>HHNKVRTCWNEGRPALAGWLQLPGTLHAEALARLDYDAVVIDMQHSPIDFGQVAPMLIAIELGGAEPFVRTQVNDPSDIMKLLDAGAYGIIAPMVNTRAEAQTLASALHYSPRGLRSFGPRRPSLRYGSGYLAQASETVVGLAMIETREALANIDEILSVDGIDGVFIGPTDLALDLGHAPLVDTEEAEVVSAIAHVRERAHAAGKRVGIWCGSGGFARVKLAEGFDFVTAAPDLAMLSAAARQVIADARAL[2x]

Here structural analysis of hydroxyketoacid aldolase from Sphingomonas wittichii RW1 (SwHKA) revealed a dynamic movement of the metal cofactor between two coordination spheres without protein scaffold rearrangements. Holo‐SwHKA forms a trimer of homodimers, in which each monomer adopts an (α/β)8 triosephosphate isomerase (TIM) barrel fold. In total, holo‐SwHKA contains six equivalent active sites; each of which is formed from amino acids from two different domain‐swapped dimers. The transition from M2+ R to M2+ A,S is induced by bidentate substrate binding and occurs without a concomitant rearrangement of the protein scaffold.

In a previous study, several variants of SwHKA were created at position F210 in order to probe the influence of aromatic electron density for CH‐π interactions with hydroxypyruvate. In the presence of ketoacids, bidentate substrate coordination affords M2+ A,S as the lowest energy complex and predominant state in crystal structures. The M2+ A,S complex is additionally stabilized by side chain interactions from the protein environment with the coordinated substrate. In particular, CH‐π interactions between the electropositive C−H bonds at C‐3 in hydroxypyruvate (HPA) and the aromatic residue F210, play an important role. Alignment of WT SwHKA M2+ A,S with monomer B from variant F210W (containing M2+ A,S/M2+ R) showed no significant change in protein structure by the F210W mutation (rmsd=0.190 Å between 243 Cα atoms).>MHIDNIENLSDREFDYIVVGGGSAGAAVAARLSEDPAVSVALVEAGP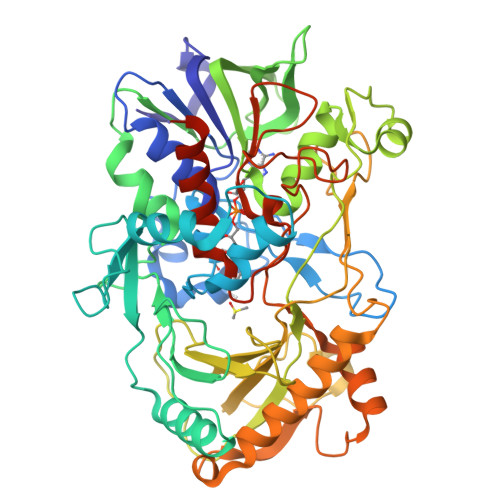DDRGVPEVLQLDRWMELLESGYDWDYPIEPQENGNSFMRHARAKVMGGCSSHNSCIAFWAPREDLDEWEAKYGATGWNAEAAWPLYKRLETNEDAGPDAPHHGDSGPVHLMNVPPKDPTGVALLDACEQAGIPRAKFNTGTTVVNGANFFQINRRADGTRSSSSVSYIHPIVEQENFTLLTGLRARQLVFDADRRCTGVDIVDSAFGHTHRLTARNEVVLSTGAIDTPKLLMLSGIGPAAHLAEHGIEVLVDSPGVGEHLQDHPEGVVQFEAKQPMVAESTQWWEIGIFTPTEDGLDRPDLMMHYGSVPFDMNTLRHGYPTTENGFSLTPNVTHARSRGTVRLRSRDFRDKPMVDPRYFTDPEGHDMRVMVAGIRKAREIAAQPAMAEWTGRELSPGVEAQTDEELQDYIRKTHNTVYHPVGTVRMGAVEDEMSPLDPELRVKGVTGLRVADASVMPEHVTVNPNITVMMIGERCADLIRSARAGETTTADAELSAALA[2x]> GAMDTRKNVSGAERKIWSLIRDCSGKLEGVTETSVLEVLLIVSRVLGIRKEDLFLKDLGVSPTEEKRILELVEKRASGYPLHYILGEKEFMGLSFLVEEGVFVPRPETEELVELALELIRKYGIKTVADIGTGSGAIGVSVAKFSDAIVFATDVSSKAVEIARKNAERHGVSDRFFVRKGEFLEPFKEKFASIEMILSNPPYVKSSAHLPKDVLFEPPEALFGGEDGLDFYR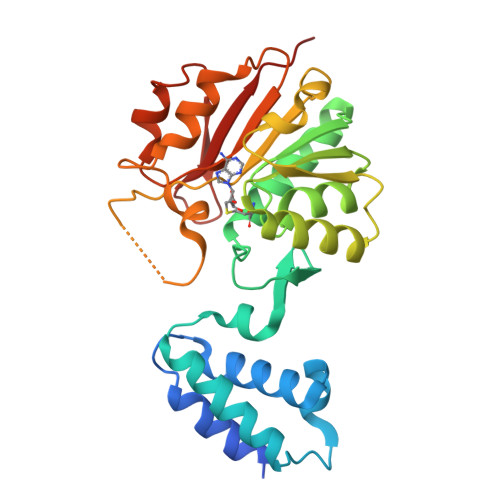EFFGRYDTSGKIVLMEIGEDQVEELKKIVSDTVFLKDSAGKYRFLLLNRRSS> MWSHPQFEKASTGREILEKLERREFTREVLKEALSINDRGFNEALFKLADEIRRKYVGDEVHIRAIIEFSNVCRKNCLYCGLRRDNKNLKRYRMTPEEIVERARLAVQFGAKTIV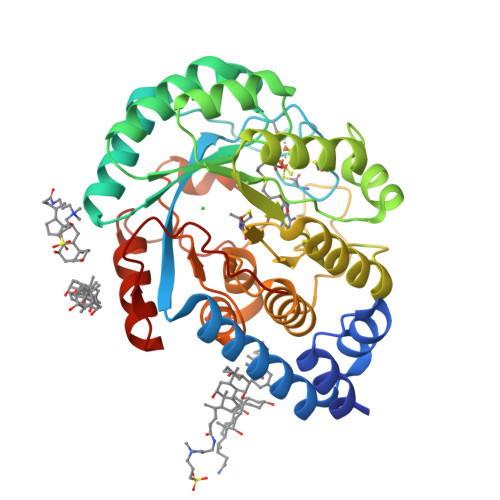LQSGEDPYXMPDVISDIVKEIKKMGVAVTLSLGEWPREYYEKWKEAGADRYLLRHETANPVLHRKLRPDTSFENRLNCLLTLKELGYETGAGSMVGLPGQTIDDLVDDLLFLKEHDFDMVGIGPFIPHPDTPLANEKKGDFTLTLKMVALTRILLPDSNIPATTAMGTIVPGGREITLRCGANVIMPNWTPSPYRQLYQLYPGKISVFEKDTASIPSVMKMIELLGRKPGRDWGGRKRVFETV>[3x]AAMALFDYNATGDTEFDSPAKQGWMQDNTNNGSGVLTN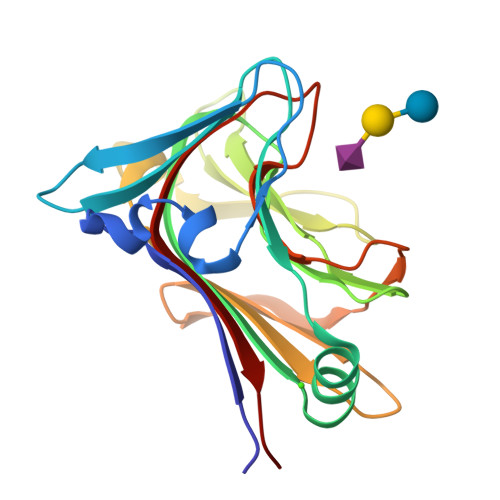ADGMPAWLVQGIGGRAQWTYSLSTNQHAQASSFGWRMTTEMKVLSGGMITNYYANGTQRVLPIISLDSSGNLVVEFEGQTGRTVLATGTAATEYHKFELVFLPGSNPSASFYFDGKLIRDNIQPTASKQNMIVWGNGSSNTDGVAAYRDIKFEIQGD> KKLAKPEKIASATSLKGSTPKAPKVFRKTEKTKHSNRKIACEASTKSSRKLTDISACSINIFYS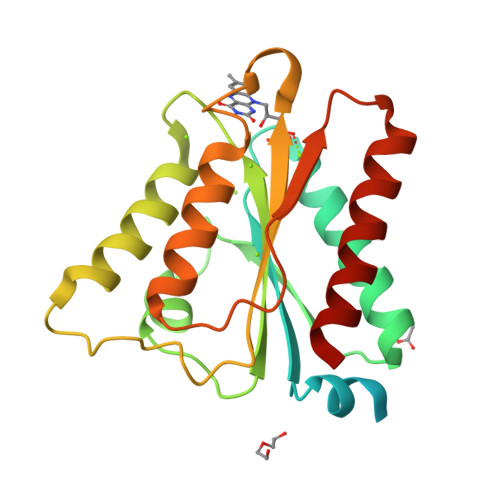TLGGSTQKFAEHVADRIRSSLQTELVEILNLDYIDLDEYFSKGNSNTVYLVLLPSYAIESSIDYFLSALQTTIDDFRIVARPLEKLRGFAVLGFGDFEQYAGDLFCYQAIAADQRLAKLGAQRIAPLGVVNVKLEKAQVYEAMEAWTDLFLQYAKEKA>[3x]MGSSHHHHHHSQDPMNQPKNIFDEIYQETEKTYRLNNIFNKLTDVEVHSYQEYSDDSKFYPSILYKDIAKTGNYTKIAIDFSFLNKNNNILIYFEKEIGPNVRVRIWNKYTRQDRTLTKSVKIALEKGDSDKYIEDETQVRAYLKKYGITAKDLDAHYEKIVNQKVLKDWCSIYKSKYSPKDYGQVTVKMQWEKW

In addition to the WXG100 protein EsxA, we demonstrated that the T7SS of S. intermedius exports three effector proteins named TelA, TelB and TelC. While the mode of action of TelA is unknown, biochemical characterization of TelB demonstrated that it exerts toxicity by degrading the electron carrying dinucleotide NAD+, whereas TelC functions as a phosphatase that cleaves peptidoglycan precursor lipid II. We have shown that TipC1 is a membrane protein with a soluble domain that localizes to the inner wall zone and is responsible for its TelC-inhibitory activity. SiB196 possesses one such tipC paralogous gene (SIR_1486), which encodes a protein with 58% identity to TipC.

In contrast to cells expressing TipC1, we found that TipC2 expression could not prevent toxicity caused by constitutive expression of the TelC toxin domain (TelCtox) targeted to the inner wall zone of SiB196 (ss-TelCtox). Crystallization efforts failed to yield diffraction quality crystals of TipC1ΔTMD or TelC–TipC1ΔTMD complex; however, TipC2ΔTMD readily crystallized in the space group C2, and we were able to determine its X-ray crystal structure to 1.8-Å resolution using selenium-incorporated protein and the selenium single wavelength anomalous dispersion technique. The resulting electron density maps allowed for complete model building of TipC2ΔTMD (residues 23–203) and a vector-encoded proline residue derived from the linker region connecting a his6-tag to the N-terminus of TipC2ΔTMD. TipC2ΔTMD adopts a mixed α/β fold consisting of three α-helices and seven β-strands that fold together to give the protein a distinct crescent-shaped appearance. This shape is characterized by a concave surface formed by a seven-stranded β-sheet and a convex surface generated by the positions of three α-helices. Using the DALI webserver to compare our structure with all deposited structures in the PDB, we determined that TipC2ΔTMD does not bear strong resemblance to proteins of known structure. The resulting TipC1ΔTMD model (residues 23–204) had a template modeling score of 0.65, indicating that the probability that our TipC1ΔTMD model has the same overall topology and fold as TipC2ΔTMD is greater than 95%. We next mapped the amino acids that vary between TipC1 and TipC2 onto the surface of the TipC1ΔTMD model, restricting our selection to amino acid R-groups with differing polarity. This analysis revealed that the majority of conserved residues are found on the convex surface, while the variable residues were predominantly found on the concave surface.> MSLGSVLNKVEDADELLKLHDLTEADLALIRKFGQIMVPKLDEYVKHFYDWLRNTPEYEQYFGDAQKLQRVQDSQVRYWKTFFDARIDSAYLKERRDVGEIHARVGLPLPTYF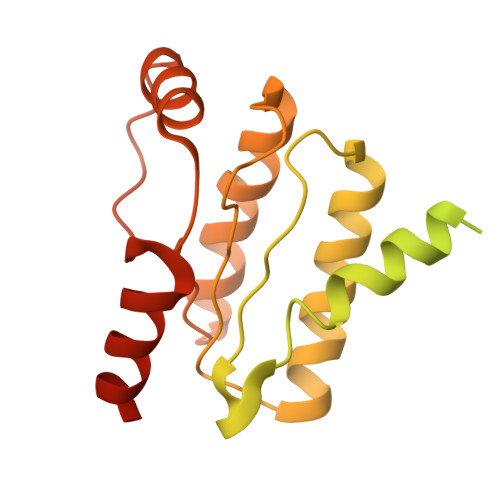AGMNISMVIFTKRMYDGSLYSDEYSSLVTAFTKLLHLDTTIVVDTYSRLINKRISEQSEALLAMSTPVTMIWQDILMLPIVGIIDSKRAQDIMSAVLNKISENRAKIFIMDISGVAVVDTAVANHFIKITKATKLMGCDCLVSGVSPSIARTMVQLGINVGEVRTNATLRDALENAFKIVGLTVSGLKHFPHE> MKVEEILEKALELVIPDEEEVRKGREAEEELRRRLDELGVEYVFVGSYARNTWLKGSLEIDVFLLFPEEFSKEELRERGLEIGKAVLDSYEIRYAEHPYVHGVVKGVEVDVVPCYKLKEPKNIKSAVDRTPFHHKWLEGRIKGKENEVRLLKGFLKANGIYGAEYKVRGFSGYLCELLIVFYGSFLETVKNARRWTRRTVIDVAKGEVRKGEEFFVVDPVDEKRNVAANLSLDNLARFVHLCREFMEAPSLGFFKPKHPLEIEPERLRKIVEERGTAVFAVKFRKPDIVDDNLYPQLERASRKIFEFLERENFMPLRSAFKASEEFCYLLFECQIKEISRVFRRMGPQFEDERNVKKFLSRNRAFRPFIENGRWWAFEMRKFTTPEEGVRSYA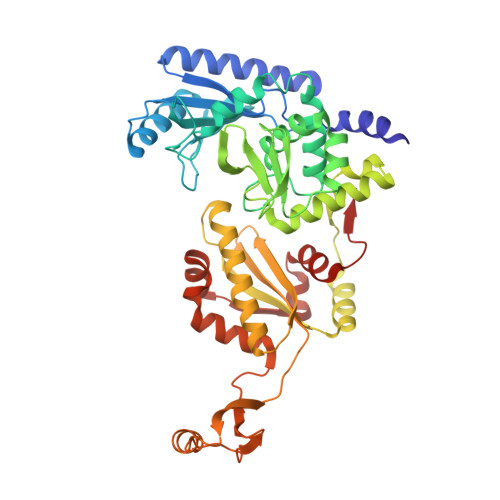STHWHTLGKNVGESIREYFEIISGEKLFKEPVTAELCEMMGVKDCCCM> MQDVQRTIEVSVGPIVGLDYTLLYDTLPETVSDNITLPDLKDPERVTEDTKKLILKGCVYIAYHHPLETDTLFIKVHKHIPEFCHSFLSHLLGGEDDDNALIDIGLFFNMLQPSL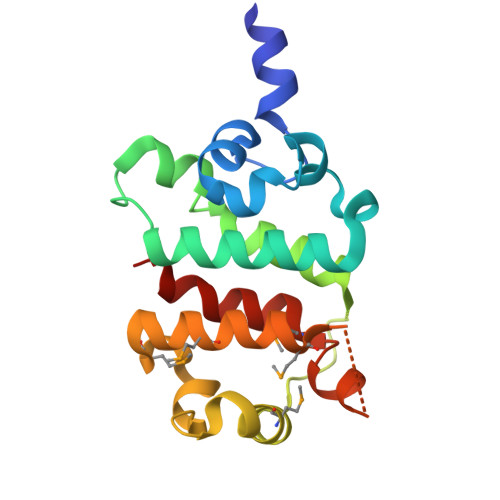GGWITKNFLRHPNRMSKDQIKMLLDQIIKMAKAESSDTEEYEKVWKKMPTYFESIIQPLLHKT Aclonifen | C12 H9 Cl N2 O3 | 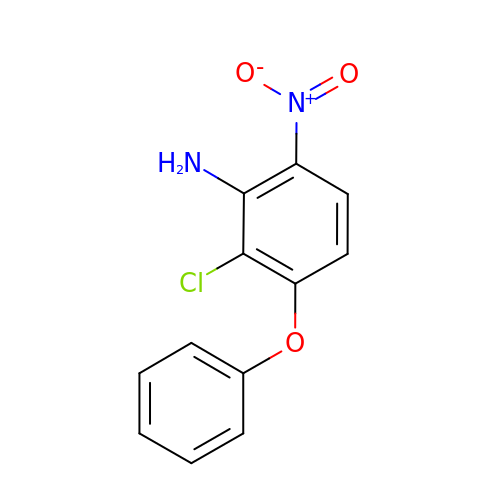DDBMQDADIHOWIC-UHFFFAOYSA-N>[4x]MAISDADLK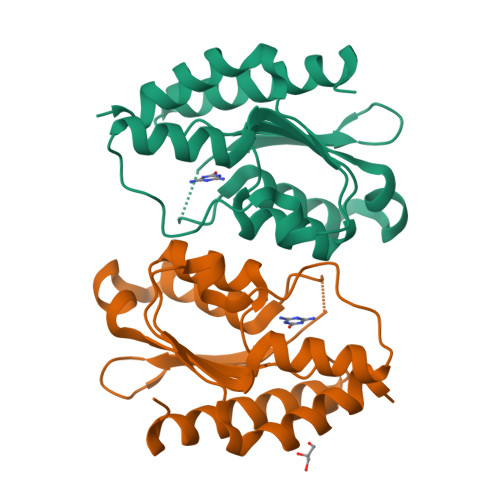YLRRCVDLAREALDDGDEPFGSVLVDHTGTTLFEDRNRVKDGDATAHPEFAIARWAARHLTPDRRARATVYTSGEHCPMCAAAHAWVGLGRIVYATSSAQLGGWLTEWGAQAPPVATLPINTVAPGVVVDGPAEELAETMHNLYRAKFGR>QVLCTNPLDIGELRSFKSKQCVDIVGNQGSGNIATYDCDGLSDQQIIICGDGTIRNEARNYCFTPDGSGNANVMSSPCTLYPEIPSSQRWRQGRRKTFTDNGGIEQVATEIINLASGKCLDIEGSDGTGDIGVYDCQNLDDQYFYVRSRGPELFYGRLRNEKSDLCLDVEGSDGKGNVLMYSCEDNLDQWFRYYENGEIVNAKSGMCLDVEGSDGSGNVGIYRCDDLRDQMWSRPNAYCNGDYCSFLNKESNKCLDVSGDQGTGDVGTWQCDGLPDQRFKWVFDDWEVPTATWNMVGCDQNGKVSQQISNTISFSSTVTAGVAVEV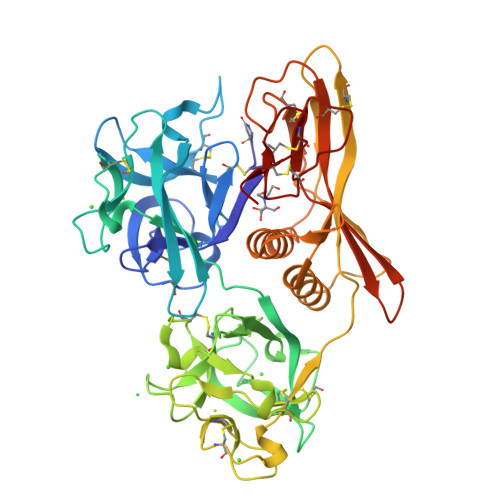SSTIEKGVIFAKATVSVKVTASLSKAWTNSQSGTTAITYTCDNYDSDEEFTRGCMWQLAIETTEVKSGDLLVWNPQIVKCTRSNTAPGCAPFTKCANEDCTFCTDI[2x]>[15x]MKSLRKMLPALLILTPLLFSPAAAEEFSASFKGTDIQEFINTVSKNLNKTVIIDPSVRGTITVRSYDMLNEEQYYQFFLSVLDVYGFAVINMNNGVLKVVRAKDAKTSAVPVASAAAPGEGDEVVTRVVPLTNVAARDLAPLLRQLNDNAGAGSVVHYEPSNVLLMTGRAAVIKRLLTIVERVDNAGDRSVVTVPLSWASAAEVVKLVTELNKDTSKSALPGSMVANVVADERTNAVLVSGEPNSRQRIIAMIKQLDRQQAVQGNTKVIYLKYAKAADLVEVLTGISSSLQSDKQSARPVAAIDKNIIIKAHGQTNALIVTAAPDVMNDLERVIAQLDIRRPQVLVEAIIAEVQDADGLNLGIQWANKNAGMTQFTNSGLPISTAIAGANQYNKDGTISSSLASALGSFNGIAAGFYQGNWAMLLTALSSSTKNDILATPSIVTLDNMQATFNVGQEVPVLTGSQTTSGDNIFNTVERKTVGIKLKVKPQINEGDAVLLEIEQEVSSVADSASSTSSDLGATFNTRTVNNAVLVGSGETVVVGGLLDKTVTDTADKVPLLGDIPVIGALFRSDSKKVSKRNLMLFIRPTIIRDRDEYRQASSGQYTAFNNAQTKQRGKESSEASLSNDLLHIYPQQETQAFRQVSAAIDAFNLGGRP;>[15x]MIHYFDYSMMRIPLIFPLCMVALLSGCQQKPASTLSPAISSQAQLEQLSSVAAGTRYLKNKCNRSDLPADETIYRAAVNVGKARGWGNIDVATLSQNSDRLYQQLLQDSTPEATQCSQFNRQLAPFIASLRSDGSDYKDDDDK;>MPVSVMRLTNINKGIIKLLPQIVTLIILITAIPQLAKLTWRVVFPVSPEDISALPLTMPPAADPELKNVRPAFTLFGLAVKNSPTPTDAASLNQVPVSSLKLRLAGLLASSNPARSIAIIEKGNQQVSLSTGDPLPGYDARIAAILPDRIIVNYQGRKEAILLFNDSRAPSPPPTAAGNPPLVKRLREQPQNILTYLSISPVLSGDKLLGYRLNPGKDASLFRQSGLQANDLAIALNGIDLRDQEQAQQALQNLADMTEITLTVEREGQRHDIAFALGDE[15x]

The protein GspD forms a 15-fold rotationally symmetric pore termed the secretin that inserts into the outer membrane (OM) and provides a conduit for substrate into the external environment. The T2SS from the human pathogen K. pneumoniae HS11286 strain comprises 13 genes in a single unidirectional operon termed PulC through to PulO. Note that Pul and Gsp nomenclature relate to equivalent proteins in homologous T2SS systems. In this study, the T2SS outer membrane components PulD and PulS are co-purified with the core components of the IM AP including PulC, PulE, PulL, PulM and PulN.

Focused refinement of the OMC yielded a reconstruction with an overall resolution of 4.3 Å. All domains of PulD were resolved with sufficient map quality to build a complete model of the monomer and the secretin, excluding the amino acids (aa) in loops 288–303, 462–470 and 632–637. The N1, N2 and N3 domains pack tightly with a diagonal offset of 36°. N0 is positioned almost directly below the N1 domain and does not maintain the diagonal offset. The N0 and N1 domains are connected by loop 7, which constitutes a substantial 26 aa linker. The N-terminus of loop 7 forms a wedge that packs between neighbouring N1 domains. The N0 domains form a tightly packed ring with alternating stacked β-sheets sandwiched between helices 2 and 4. Importantly, each PulC HR domain binds to only a single PulD N0 domain and has no contact with neighbouring PulC HR domains. Overall, the binding of the PulC HR domain to the PulD N0 domain appears to be important for the correct positioning of the N0 domain within the secretin and the subsequent stabilisation of the N1 and N2 domains. Loop 38 between S-domain helix 14 and helix 15 bound to PulS constitutes the lone contact point between the secretin core and PulS.>MMQQSRPASDPQVVEAARKEGRLIIYSATDQSSAQALLDDFRKLYPFIQIEYNDL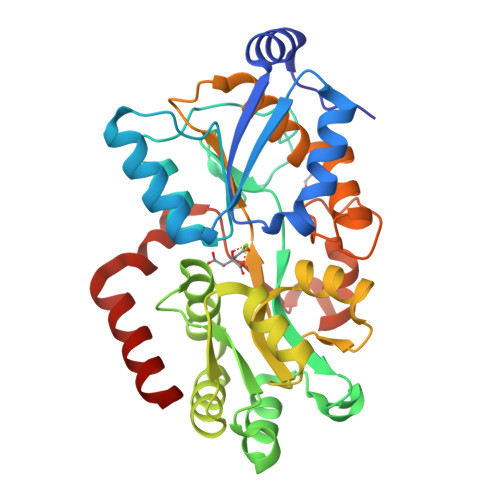GTQAIYDRFVSETAAGASSADLLWSSAMELQVKLASEGYALPYDSPEAKNWPANARLGNLAYSTTLEPAVVVYNKRFLKPEEVPTTREGLARLLQEPRMRGRVATWDPERSAVGFTILKADYDRFPAFQELARAFGKAQAALYSSTGAAFEKVISGEHYLAYGFFGSYALLRQRTVKDLGIAYLTDGTVAIQRVAFINKRAAHPNAAKLFLDYLLSLRGQNLMAYTALIFARRETVVGEATPQALYKAVGGKDKVYAIPVSTEILKNLDPAERMRFLTFWRQAVRGQ[3x]>MFQCNVPLGMESGRIANEQISASSTYSDGRWTPQQSRLHGDDNGWTPNLDSNKEYLQVDLRFLTMLTAIATQGAISRETQNGYYVKSYKLEVSTNGEDWMVYRHGKNHKVFQANNDATEVVLNKLHAPLLTRFVRIRPQTWHSGIALRLELFGCRV[4x];>SCKNTDSRCKARQLELNERT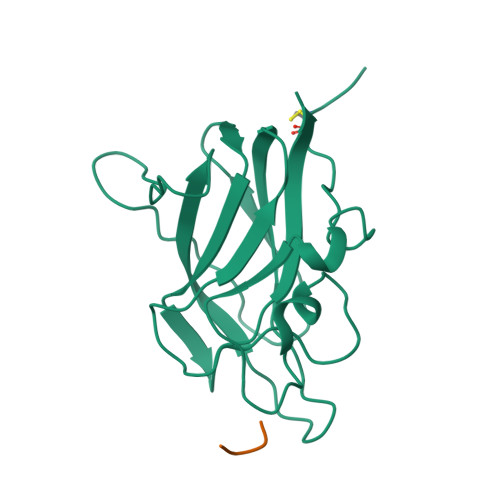CRCDKPRR[3x]> GTGADP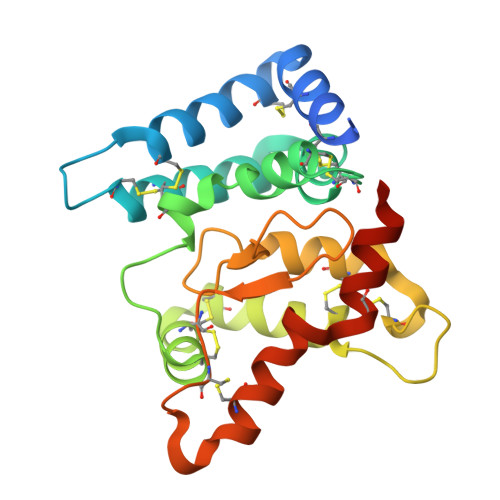VVSAKSNHCLDAAKACNLNDNCKKLRSSYISICNREISPTERCNRRKCHKALRQFFDRVPSEYTYRMLFCSCQDQACAERRRQTILPSCSYEDKEKPNCLDLRGVCRTDHLCRSRLADFHANCRASYQTVTSCPADNYQACLGSYAGMIGFDMTPNYVDSSPTGIVVSPWCSCRGSGNMEEECEKFLRDFTENPCLRNAIQAFGNGTDVN>[2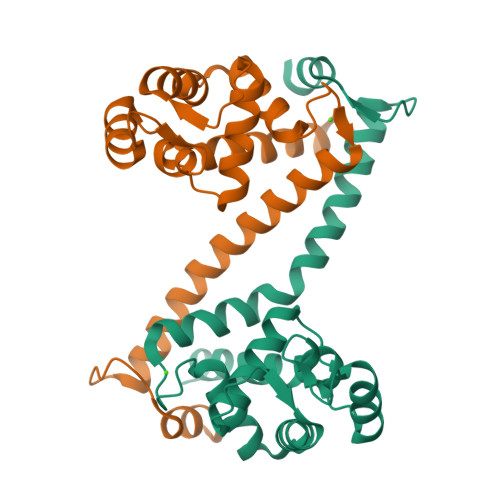x]AMGTKSSAAVALKGLQFVTAKVGNDGWAAVEKRFNQLQVDGVLLRSRFGKCIGMDGSDEFAVQMFDSLARKRGIVKQVLTKDELKDFYEQLTDQGFDNRLRTFFDMVDKNADGRLTAEEVKEIIALSASANKLSKIKERADEYTALIMEELDPTNLGYIEMEDLEALLLQSPSEAAARS There has been considerable interest towards an improved understanding of the cleavage mechanisms that underlie RNA catalysis by small self-cleaving ribozymes involved in self-scission during rolling circle replication of viral genomes. Such challenges are highlighted by the recent identification of a new set of self-cleaving ribozymes from genomic bioinformatics searches, named twister, twister-sister, pistol, and hatchet ribozymes. We report here the structure of a four-way junctional twister-sister ribozyme and discuss possible/putative roles of selected nucleobases and hydrated Mg2+ ions observed at the active site for cleavage chemistry. For crystallographic studies, we introduced dC62 into the sequence of the longer substrate strand of the two-stranded construct, so as to prevent cleavage at the known C62–A63 cleavage site of the twister-sister ribozyme.

There are two molecules of the twister-sister ribozyme in each asymmetric unit (space group: P21212), with both exhibiting well-defined electron density, while also superpositioning well with an rmsd = 0.27 Å. As shown in the schematic of the tertiary fold of our construct of the twister-sister ribozyme, stems P1, P2, and P3 form one continuous helix, whereas stems P4 and P5 form a second continuous helix, with elements of these two continuous helices meeting at the junctional site. Notably, SL4 projecting from continuous helix P5–P4 is positioned in the minor groove of the partially zippered-up L1 loop segment associated with the continuous helix P1–P2–P3 helix. We have observed a large number of binding sites for hydrated metal cations in the structure of the twister-sister ribozyme, with the focus in this paper on metal sites labeled M1 to M7, positioned either at the junctional or cleavage sites. At the junctional site of the twister-sister ribozyme, both splayed-apart C24–G25 (junctional J34 segment) and G55–G56 (junctional J52 segment) steps are brought into close proximity, with a hydrated Mg2+ (labeled M5) bridging opposingly aligned J34 and J52 junctional segments. Bases C62 and A63 at the cleavage site are splayed apart, with C62 directed outwards and A63 directed inwards into the ribozyme fold. C62 appears to adopt a mixture of syn and anti conformations reflective of flexibility about its glycosidic bond, whereas A63 is anchored in place in an anti conformation by stacking between bases, with its N7 atom hydrogen bonded to the 2′-OH of C6. The hydrated octahedrally coordinated Mg2+ cation M2 is positioned to form an inner-sphere coordination to the modeled 2′-O of C62 at the cleavage step. There are no base or sugar residues within hydrogen bond distance of the 2′-O of C62 and hence hydrated M2 could be a potential candidate for activation of the 2′-OH of C62, as suggested previously. Finally, off-line cleavage alignments are observed both in the 4-wj structure (O2′ P-O5′ angle of 71°) and in the 3-wj structure (67°)17 for the pre-catalytic state of the twister-sister ribozyme.

>[2x]ACCCGCAAGGCCGACGGC;>[2x]GCCGCCGCUGGUGCAAGUCCAGCCACGCUUCGGCGUGGGCGCUCAUGGGU> GNDEQEVNMVKPTNANSEIEVINDGTMIKFKDVESYENALLKVSAMSTSEQVSFLNSLSFKSQMILMQEADGELDKICNQA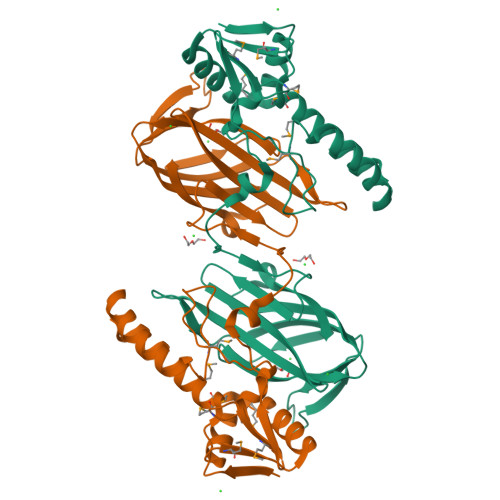ADKAEFDVLYEKYKHKYGDVFMFNTIDATDLSPYSRLVYVANEYFVNMKGEFMIGDSLVVDKVYTDFKERQQQFTVSTRSSVSDLSSINEAYSRQKDRKVGLYLSVSSGIIHANFTSQKKGVFGWSRYSTTYHAKVNLRGFEFAQGELLGYGPVYVNKDGIPFAIDTKEMGGNVTKVFGRKLAQECTGTIEIWSRGVPYDQRGFATVRL>ADQRRDFIDIESKFALRTPEDTAEDTCHLIPGVAESVATCHFNHSSKTFMVIHGWTVTGMYESWVPKLVAALYKREPDSNVIVVDWLSRAQEHYPVSAGYTKLVGQDVARFINWMEEEFNYPLDNVHLLGYSLGA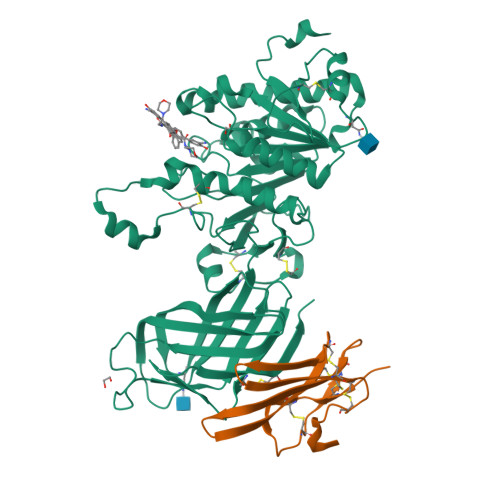HAAGIAGSLTNKKVNRITGLDPAGPNFEYAEAPSRLSPDDADFVDVLHTFTRGSPGRSIGIQKPVGHVDIYPNGGTFQPGCNIGEAIRVIAERGLGDVDQLVKCSHERSIHLFIDSLLNEENPSKAYRCSSKEAFEKGLCLSCRKNRCNNLGYEINKVRAKRSSKMYLKTRSQMPYKVFHYQVKIHFSGTESETHTNQAFEISLYGTVAESENIPFTLPEVSTNKTYSFLIYTEVDIGELLMLKLKWKSDSYFSWSDWWSSPGFAIQKIRVKAGETQKKVIFCSREKVSHLQKGKAPAVFVKCHDKSLNKKSG[4x];>[4x]QTQQEEEEEDEDHGPDDYDEEDEDEVEEEETNRLPGGRSRVLLRCYTCKSLPRDERCDLTQDCSHGQTCTTLIAHGNTESGLLTTHSTWCTDSCQPITKTVEGTQVTMTCCQSSLCNVPPWQSSRVQDPTG During bacterial cell growth, hydrolases cleave peptide cross-links between strands of the peptidoglycan sacculus to allow new strand insertion. The Pseudomonas aeruginosa carboxyl-terminal processing protease (CTP) CtpA regulates some of these hydrolases by degrading them. CtpA assembles as an inactive hexamer composed of a trimer-of-dimers, but its lipoprotein binding partner LbcA activates CtpA by an unknown mechanism. LbcA has an N-terminal adaptor domain that binds to CtpA, and a C-terminal superhelical tetratricopeptide repeat domain.

The LbcA density in the CtpA–LbcA EM map thickens in the middle of the TPR region, suggesting that the TPR domain may fluctuate in multiple conformations. Therefore, we performed a heterogeneous refinement leading to two CtpA–LbcA EM maps. As expected, the two CtpA hexamers in the two 3D maps are superimposable but the two LbcA supercoils are wide apart, with one supercoil in a higher position remote to the front CtpA and the other in a lower position proximal to the front CtpA. We next performed focused refinement in the top one-third region of the two maps and derived two local EM maps at around 4 Å resolution. We found that in these two local structures, the LbcA adaptor domain (H1–H6) binds to CtpA in essentially the same binding mode, and the difference between the two structures is limited to the LbcA TPR domain, which is 44 Å and 18 Å, respectively, above the front CtpA. In the proximal binding mode, the LbcA hinge region (H7–H8) rotates clockwise by 26°, compared to the hinge region in the remote mode, to lower the TPR domain by 22 Å and orient it towards, but apparently not contact, the substrate binding pocket of the front active CtpA. TPRs often serve as a scaffold to mediate protein–protein interaction. Therefore, we suggest that the observed TPR domain movement might be linked to substrate protein binding and delivery to the CtpA proteolytic site. However, both conformations were in complex with active CtpA, implying that the two positions of the superhelical TPR domain have no effect on the allosteric activation mechanism.

>[3x]GSHMSAPLPLDELRTFAEVLDRVKAAYVEPVDDKTLLENAIKGMLSNLDPHSAYLGPEDFAELQESTSGEFGGLGIEVGSEDGFIKVVSPIDDTPAARAGIQPGDLIVQIDGKPTKGQSMTEAVDSMRGKAGSPITLTIVRDGGRPFDVELKRAIIKVKSVKSQVLEPGYAYLRITQFQVNTGEEVVKALNQLRKDNKGRLKGLVLDLRNNPGGVLQSAVEVADAFLTKGLIVYTKGRIANSELRFSADPADPSDKVPLVVLINGGSAAAAEIVAGALQDQKRAILMGTDSFGKGSVQTVLPLNNDRALKLTTALYYTPNGRSIQAQGIVPDIEVGRAKVTQERSSFEGFKEADLQGHLANGNGGADRPTGKRAAPSERPQDSDYQLSQALSLLKGLSVTRGN;> MEDTAVETKAKPEKYGSFSEDSLYSLLVAELAGQRNRFDIALSNYVVQAQKTRDPGVSERAFRIAEYLGADQEALDTSLLWARSAPDNLDAQRAAAIQLARAGRYEESMVYMEKVLNGQGDTHFDFLALSAAETDPDTRAGLLQSFDHLLKKYPNNGQLLFGKALLLQQDGRPDEALTLLEDNSASRHEVAPLLLRSRLLQSMKRSDEALPLLKAGIKEHPDDKRVRLAYARLLVEQNRLDDAKAEFAGLVQQFPDDDDLRFSLALVCLEAQAWDEARIYLEELVERDSHVDAAHFNLGRLAEEQKDTARALDEYAQVGPGNDFLPAQLRQTDVLLKAGRVDEAAQRLDKARSEQPDYAIQLYLIEAEALSNNDQQEKAWQAIQEGLKQYPEDLNLLYTRSMLAEKRNDLAQMEKDLRFVIAREPDNAMALNALGYTLADRTTRYGEARELILKAHKLNPDDPAILDSMGWINYRQGKLADAERYLRQALQRYPDHEVAAHLGEVLWAQGRQGDARAIWREYLDKQPDSDVLRRTIKRLTGAETP> TGYLTIGGQRYQAEINDLENLGEMGSGTCGQVWKMRFRKTGHVIAVKQMRRSGNKEENKRILMDLDVVLKSHDCPYIVQCF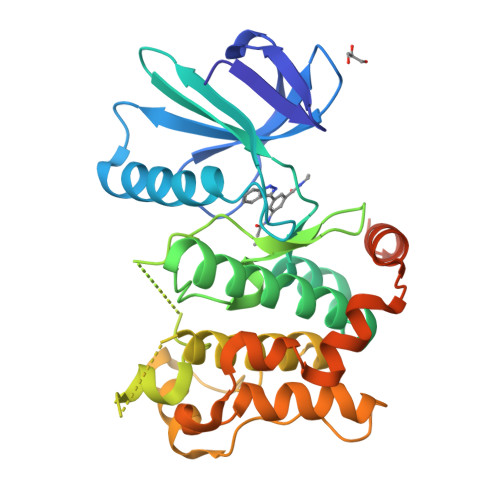GTFITNTDVFIAMELMGTSAEKLKKRMQGPIPERILGKMTVAIVKALYYLKEKHGVIHRDVKPSNILLDERGQIKLCDFGISGRLVDSKAKTRSAGCAAYMAPERIDPPDPTKPDYDIRADVWSLGISLVELATGQFPYKNCKTDFEVLTKVLQEEPPLLPGHMGFSGDFQSFVKDCLTKDHRKRPKYNKLLEHSFIKRYETLEVDVASWFKDVMAKTESPRTSGVLSQPHLPFFRHHHHHH> MAYSDYSDGADDMPDFHDEGEFDDYLNDDEYELMNEVFPTLKAQLQDYQGWDNLSLKLALFDNNFDLESTLAELKKTLKKKKTPKKPIAAANGSANVTQKLANISISQQRPNDRLPDWLDEEESEGERNGEEANDEKTVQRYYKTTVPTKPKKPHDISAFVKSALPHLSFVVLGHVDAGKSTLMGRLLYDLNIVNQSQLRKLQRESETMGKSSFKFAWIMDQTNEERERGVTVSICTSHFSTHRANFTIVDAPGHRDFVPNAIMGISQADMAILCVDCSTNAFESGFDLDGQTKEHMLLASSLGIHNLIIAMNKMDNVDWSQQRFEEIKSKLLPYLVDIGFFEDNINWVPISGFSGEGVYKIEYTDEVRQWYNGPNLMSTLENAAFKISKENEGINKDDPFLFSVLEIIPSKKTSNDLALVSGKLESGSIQPGESLTIYPSEQSCIVDKIQVGSQQGQSTNHEETDVAIKGDFVTLKLRKAYPEDIQNGDLAASVDYSSIHSAQCFVLELTTFDMNRPLLPGTPFILFIGVKEQPARIKRLISFIDKGNTASKKKIRHLGSKQR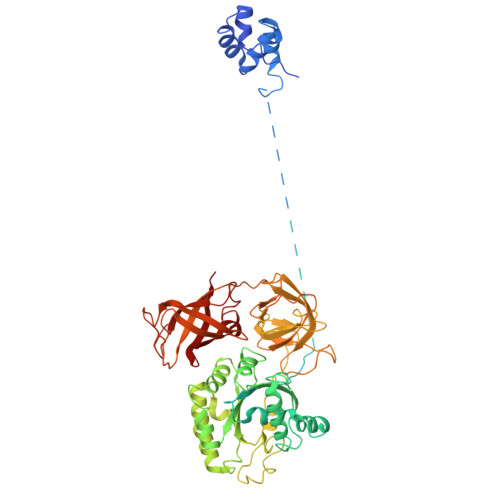AFVEIELIEVKRWIPLLTAHENDRLGRVVLRKDGRTIAAGKISEITQ>[6x]SNATKKSAAEASKKPRQKRTATKAYNVTQAFGRRGPEQTQG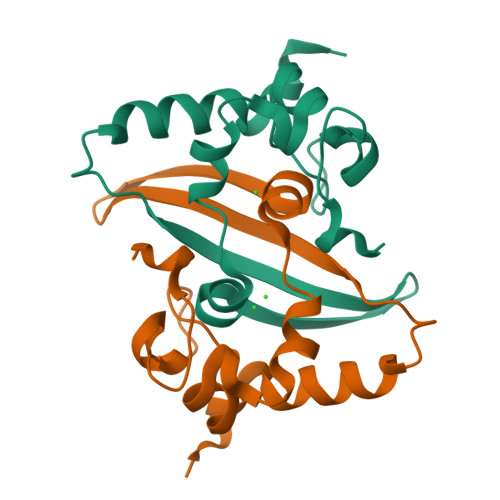NFGDQELIRQGTDYKHWPQIAQFAPSASAFFGMSRIGMEVTPSGTWLTYTGAIKLDDKDPNFKDQVILLNKHIDAYKTFP> ADPPAPSTRRPPAPNLHVSPELFCEPREVRRVQWPATQQGMLVERPCPKGTRGIASFQCLPALGLWNPRGPDLSNCTSPWVNQVAQKIKSGENAANIASELARHTRGSIYAGDVSSSVKLMEQLLDILDAQLQALRPIERESAGKNYNKMHKRERTCKDYIKAVVETVDNLLRPEALESWKDMNAT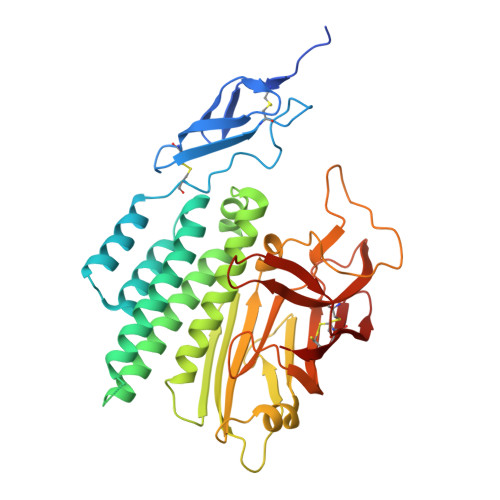EQVHTATMLLDVLEEGAFLLADNVREPARFLAAKQNVVLEVTVLSTEGQVQELVFPQEYASESSIQLSANTIKQNSRNGVVKVVFILYNNLGLFLSTENATVKLAGEAGTGGPGGASLVVNSQVIAASINKESSRVFLMDPVIFTVAHLEAKNHFNANCSFWNYSERSMLGYWSTQGCRLVESNKTHTTCACSHL> SKYGLQDSDEEDDQLNNAEAKKLKAAPVPPQGKPPPLQQATLPGKVTPPPQSPAVDQLDRVLELDSDMADITQDQDLDSVAEEQDITEEQEPLSASSHIASSLGINPHALQVMKASLLLEEEDGEMINRFSSFPSSMDPYPDVRSPRLFPSSHAKRTSSMGLLQSKFASPSISRISETAQGSHSPRILPVTPWSVPAPLAPTFVIPRPAPETHLRTVGTRRQQELVPLEKSVTHGRGSLLIDMGLFMGRSFRVGWGPNWTLVHNGDKLTERLNAEEDQNMDTIDYGFLPKPTSAKSLTESPFKVHMEKLSLEQKSRELQSYLMPLEIELKNSSVDRSAQCPHFKPNAGVAAIHDYAGWVRNLSNEAGELEAVVKQWGLTWTLCESLWGQLKELEASLDEPNEYVRNLERRKAFSHWLAHTAEERIEEEVSLYGPERHVEAVFSFLTGGRISDACRLAQKSGDHRLSLLLSQMVGSQEMRELISLQLVDWNKLQVDHYIQEERLRVFCLLSGTPVWRSSDNRSINVCSQLDWKRTLAVHLWYMLPPTATIAQALRLYERAFQEHEEGEPYACYPLP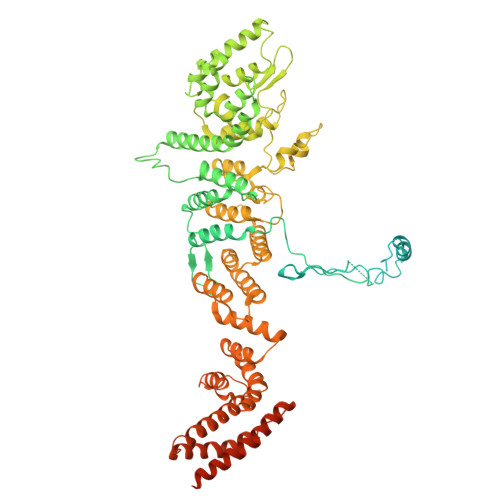PYLEDCSISLGDEPSAKFSSLQRDVCVHLLKLYSERQYDLCQLLDPSSVTPDPLDYRLSWHLWMVLQALNYTHLSEHRQGTLHASYAAQLENVGLWEWAIFVLLHIPHPHIREAGVRELLNRQCVVRESPESLAKENFLIHRLCVPAQWVHEAKAIRSRRDGDRHKEALYLLKGHQWNPCHKLVTRHLAADAVINENYRYLQSFLGELSNPEHCKHIQDWETAGKVYLDYIRVIDMLNLIQQDESSGCELEKLHTKVMSLCKWVELIHCYTAKDRLAQSEMAKRVANILRVVLSLQQPPESMSDSSEPRVPLRLLAPHIGRLPMPEDYALEELRGLTQSYLRELICDS> MKDLLKFLKAQTKTEEFDAIKIALASPDMIRSWSFGEVKKPETINYRTFKPE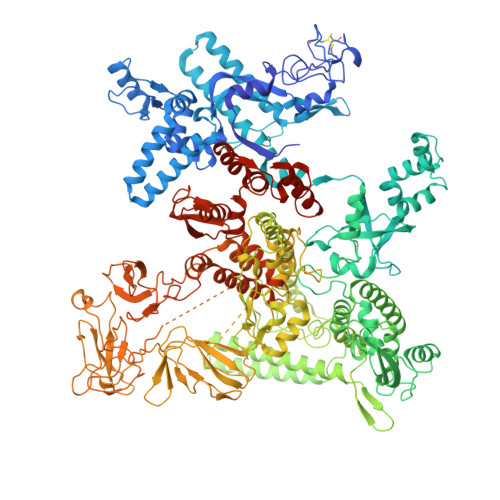RDGLFCARIFGPVKDYECLCGKYKRLKHRGVICEKCGVEVTQTKVRRERMGHIELASPTAHIWFLKSLPSRIGLLLDMPLRDIERVLYFESYVVIEGGMTNLERQQILTEEQYLDALEEFGDEFDAKMGAEAIQALLKSMDLEQECEQLREELNETNSETKRKKLTKRIKLLEAFVQSGNKPEWMILTVLPVLPPDLRPLVPLDGGRFATSDLNDLYRRVINRNNRLKRLLDLAAPDIIVRNEKRMLQEAVDALLDNGRRGRAITGSNKRPLKSLADMIKGKQGRFRQNLLGKRVDYSGRSVITVGPYLRLHQCGLPKKMALELFKPFIYGKLELRGLATTIKAAKKMVEREEAVVWDILDEVIREHPVLLNRAPTLHRLGIQAFEPVLIEGKAIQLHPLVCAAYNADFDGDQMAVHVPLTLEAQLEARALMMSTNNILSPANGEPIIVPSQDVVLGLYYMTRDCVNAKGEGMVLTGPKEAERLYRSGLASLHARVKVRITEYEKDANGELVAKTSLKDTTVGRAILWMIVPKGLPYSIVNQALGKKAISKMLNTCYRILGLKPTVIFADQIMYTGFAYAARSGASVGIDDMVIPEKKHEIISEAEAEVAEIQEQFQSGLVTAGERYNKVIDIWAAANDRVSKAMMDNLQTETVINRDGQEEKQVSFNSIYMMADSGARGSAAQIRQLAGMRGLMAKPDGSIIETPITANFREGLNVLQYFISTHGARKGLADTALKTANSGYLTRRLVDVAQDLVVTEDDCGTHEGIMMTPVIEGGDVKEPLRDRVLGRVTAEDVLKPGTADILVPRNTLLHEQWCDLLEENSVDAVKVRSVVSCDTDFGVCAHCYGRDLARGHIINKGEAIGVIAAQSIGEPGTQLTMRTFHIGGAASRAAAESSIQVKNKGSIKLSNVKSVVNSSGKLVITSRNTELKLIDEFGRTKESYKVPYGAVLAKGDGEQVAGGETVANWDPHTMPVITEVSGFVRFTDMIDGQTITRQTDELTGLSSLVVLDSAERTAGGKDLRPALKIVDAQGNDVLIPGTDMPAQYFLPGKAIVQLEDGVQISSGDTLARIPQESGGTKDITGGLPRVADLFEARRPKEPAILAEISGIVSFGKETKGKRRLVITPVDGSDPYEEMIPKWRQLNVFEGERVERGDVISDGPEAPHDILRLRGVHAVTRYIVNEVQDVYRLQGVKINDKHIEVIVRQMLRKATIVNAGSSDFLEGEQVEYSRVKIANRELEANGKVGATYSRDLLGITKASLATESFISAASFQETTRVLTEAAVAGKRDELRGLKENVIVGRLIPAGTGYAYHQDRMRRRAAGEAPAAPQVTAEDASASLAELLNAGLGGSDNE In this work, we set out to find the physiological substrate of the cofactor-independent racemase (predicted DapF, FN1732) from F. nucleatum ATCC 25586, and were surprised to find that this enzyme functions as a histidine racemase (HisR). Here, we characterize this enzyme as a histidine racemase (HisR), and found that catalytic turnover is ∼10,000× faster with L-histidine than with L,L-lanthionine. The rate of HisR was not affected by buffer composition (PO4 or Tris), ions (SO42−, Mg2+, and EDTA), or the PLP inhibitor hydroxylamine; however, the enzyme activity was hindered by iodoacetamide and Hg2+, which are known inhibitors of enzymes with catalytic thiols. These results, along with a sequence alignment of HisR with other cofactor-independent racemase and epimerase enzymes, suggested that HisR operates via a two-base mechanism using cysteine residues 67 and 209. The DapF-like fold is an overall α+β structure, in which the monomer unit is composed of two structurally equivalent N-terminal and C-terminal domains.

To confirm this, we used site-directed mutagenesis to generate HisR mutants C67S and C209S. Catalytic turnover of these mutants was greatly reduced with D- and L-histidine compared to the WT enzyme, as expected. Mutation of an active site cysteine to serine is a common strategy to aid crystallization of cofactor-independent epimerases and racemases, and likely aids the process because this mutation slows catalysis and helps to keep the enzyme in the open conformation. In the asymmetric unit of C67S, there are two back-to-back dimers, while the asymmetric unit of C209S has one dimer and two monomers. Structures of C67S and C209S HisR were very similar, with a backbone r.m.s.d. of 0.493 Å by aligning α-carbons of 260 residues, and each adopt a DapF-like fold. In each structure, a sulfate (mutant C67S) or a phosphate (mutant C209S) is found in the active site directly between catalytic residues. Catalytic residues 67 and 209 reside at the N-terminal ends of central α-helices 2 and 4, allowing for stabilization of the negative charge formed on cysteine thiolates by helix dipoles during the reaction. The position of the loops above the active site spanning from residues 42 to 49 (N-terminal domain) and 197 to 206 (C-terminal domain) in HisR more closely match the conformation of the open C. glutamicum structure than the substrate-bound, closed form. CntK and other enzymes with a DapF-like fold are typically functional as homodimers, and HisR appears to maintain this feature.

>MDRKVQVLDFIKINPAGNITILIDNFDIYDKNIPKLSEEIMKETNLYAEQVGFIKDSHLQMMGGEFCGNASRAFASLLAFRDKDFSKQKNYNITCSGESKVLDVDVRNDGAKNKFLAKIKMPKFLSLEEINVDEYKLGLVRFSGINHFIFNIKENKETSFENIIDLVKKYLSNEEYSAFGIMFFDSDNLSMKPYVYVKEVGSGVYENSSASGTTALGYYLKKCKNLDRAKIVQPNGWLEYIIENDEMYIDGPVEIIAEGKIYIGKHHHHHH[4x]>ETLVRPKPLLLKLLKSVGAQKDTYTMKEVLFYLGQYIMTKRLYDEKQQHIVYCSNDLLGDLFGVPSFSVKEHRKIYTMI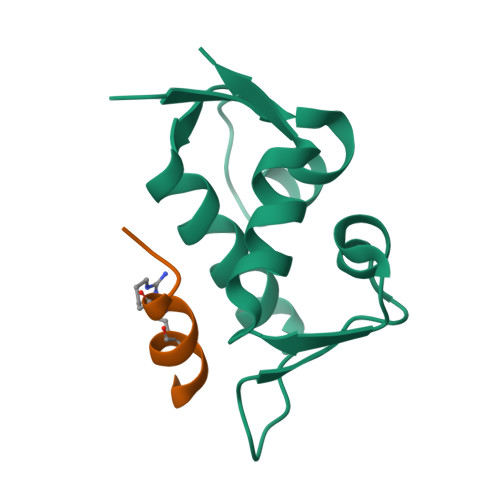YRNLVVV[4x];>XTSFLEYWRLLSPX[3x]> GPMPGKKFVARVAEARAEDVGKRVVIIPKAERAKVGIKVGDVVEVKKV

Here, we study fold transition between distinct β-barrels by protein engineering and structural biology technique. Here, we discover that the previously reconstructed ancient DPBB sequence could also adopt a β-barrel fold named Double-Zeta β-barrel (DZBB), as a metamorphic protein. The DZBB fold is not found in any modern protein, although its structure shares similarities with RIFT and OB. Furthermore, the reconstructed OB fold could also be converted to the four-stranded SH3 fold by a simple circular permutation. Thus, these ancient β-barrel folds (DPBB, RIFT, OB, and SH3) could be readily interconverted by a few feasible mutations through the missing-link fold, DZBB, indicating their significantly close evolutionary relationships.

Phs018 has remarkable sequence similarity to design-1 (26–35% identity), and we replaced five residues in design-1 with the ones at the corresponding positions of Phs018. AlphaFold2 (AF2)19 predicted that the resultant mutant, design-2 (Ph1), would fold into a RIFT-like structure, albeit with a low lDDT region in the 1st β-turn. Circular dichroism (CD) and size exclusion chromatography (SEC) experiments indicated that design-2 was folded (not random coil) and had moderate stability (Tm = 58 °C). Design-2 also formed crystals under similar buffer conditions to the third type of design-1 crystal, including lithium sulfate. By molecular replacement with the predicted design-2 model (RIFT fold) and subsequent manual remodeling, the crystal structures of design-1 (third type of crystal) and design-2 were determined. Surprisingly, they both adopted into a unique β-barrel fold that topologically differs from DPBB and RIFT. The five point-mutations derived from Phs018 (RIFT) in design-2 stabilized the DZBB fold. Furthermore, the addition of five-point mutations in design-2 stabilized the DZBB fold and abolished the capability to adopt the DPBB fold. Most DNA molecules did not migrate from the well when mixed with the proteins with the stable DZBB fold (design-2, -18, and -19) and RIFT fold (design-3 and -4), indicating that these proteins formed large aggregates with dsDNA. Design-2 seems to have a higher affinity for dsDNA than design-3, as dsDNA shifted even at lower concentrations of design-2.Cdc23 is one subunit of the multimeric anaphase-promoting complex (APC/C) which controls sister-chromatid segregation and the exit from mitosis by mediating the ubiquitin-dependent degradation of cell-cycle regulatory proteins. The Cdc23Nterm subunit has 282 residues, with six cysteines and five methionines (one S atom per 25 residues), and is thus comparable in size and sulfur content to the lysosomal protein from mouse solved using S-SAD by Lakomek et al.. The sequence identity of Cdc23Nterm to other proteins is below 30%, making difficult to find models in the PDB for molecular replacement. In this paper, we report the structure solution of Cdc23Nterm achieved at P13 using a S-SAD experiment at λ = 2.69 Å (4.6 keV) and the related methods and we discuss the instrumentation.

The wavelength was chosen to maximize the Bijvoet ratio, on the basis of the available energy range at the beamline and the expected diffraction resolution of the sample, following the decision-making model for an S-SAD experiment proposed by Cianci et al.. TRUNCATE and PHENIX confirmed the presence of merohedral twinning with twin law (h, −k, −l) with an estimated twin fraction of 0.37. Clearly, the two halves of the crystal were actually two separate crystalline domains and were successfully treated as such. A variable micrometre-size beam allowed the collection of sulfur data from separate regions of a crystal, which would otherwise be discarded, thus overcoming crystal imperfections owing to the presence of two differently oriented twin domains. The long wavelength enhanced the Bijvoet ratio to 2.21% (1.0% at 7 keV), thus increasing the anomalous signal to a level where it was possible to determine the sulfur substructure accurately even with moderate data multiplicity. The quality of the calculated phases allowed the autotracing of 384 of the final 472 rebuilt residues (81%) at 3.1 Å resolution. The Cα r.m.s. deviations, calculated with LSQKAB for 219 residues, between this structure and that reported by Zhang et al. are 0.80 and 0.92 Å for chain A and chain B, respectively.

>[2x]MQLREIRNCLLKCISECSERGLVYAVRWAAEMLNGMNPIEMEHIPFSSTPTGEFDLDPDMANEKLLEVEEKNIYLLAKSYFDCKEFERAAYTLQNCKSSKSIFLRLYSKYLAGEKKSEEENETLLNTNLTLSSTNREFYYISEVLESLHYQGNKDPYLLYLSGVVYRKRKQDSKAIDFLKSCVLKAPFFWSAWLELSLSIDSLETLTTVVSQLPSTHIMTKIFYVYASHELHQVNSSAYEKLAEAEIIFPNSRYLKTQRALLTYDSRLFDEAESLFENILTNDPAENLYFQ> SLAGETINFCKGWKFHLGDAGKGASSSSYNDSQWRILNIPHDWSIEGTYKQFENGTDWQSGFLPAGISWYRKTFTIPSKWKNKKVQILFEGVYLNSEVWINGHWLGKRPNGYISFVYDLTPYLQEGKNQIAVKVDHSKALTGRWYTGSGIYRPVYLLVSNPTHIPYSGIHFRSKLQNKQSATYTLSIEIETQEKKPIKVKTYLQAPNGSIADTSEKIFVSSADSLCFLSGSIRKPLLWSPDSPNVYTLICQLTRDNKILDECRLPVGFRQLEFNPVSGFLLNGKSLKIKGVCDHHTVGAVGAAVPDDLLHYRLKLLKDMGCNAIRTSHNPFSPAFYNLCDTMGIMVLNEGLDGWNQPKAADDYGNYFDEWWQKDMTDFIKRDRNHPSIIMWSIGNEVTGATPEIQHNLVSLFHQLDPDRPVTQGGTDPTRGMKTDYQKKFNYLDIIGFNGNGEEIGELEHFHKNYPTLCAIATEVPHTYQTRGVYRSQTQWRRRDFPAPWEKGNINWEQFKHRVFPIPDLTEKECFPEESDYPYYQSSYDNASVRISARKSWQRTCSFPWLMGEFRWGSFDYLGEAEWPQRCGNFGIIDIA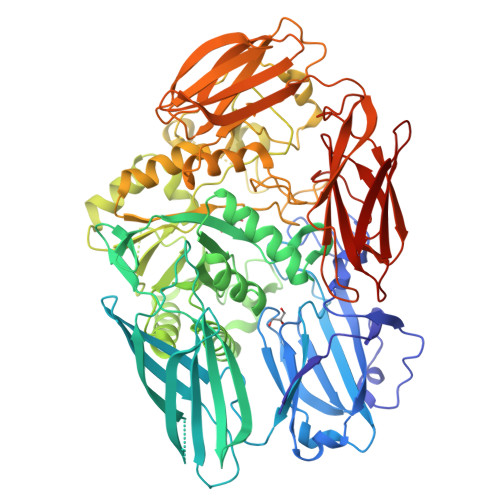AIPKDAYFLYQSLWTDKPMVHLLPHWTHPGKEGKTIPVVIYTNCDAVELFINNVSLGSKPYTGEQLIWLVPYSPGKIEARGIKKGKIVATDCYQSAEAPHSVALASNKYSVKAGSDEVIRIEIDITDKNGIPCPYASNELSFHVSGPLRLLGVDNGNPTDMFPYQQPHCRCFRGKCVVLLQSDEEKGKGTLTVQGTKLVEKKLIIEVIEG>MGSSHHHHHHSSGLVPRGSHMPSYTVTVATGSQEHAGTDDYIYLSLVGSAGCSEKHLLDKGSFERGAVDSYDVTVDEELGEIQLVRIEKRKYGSNDDWYLKYITLKTPHGDYIEFPCYRWITGDVEVVLRDGRAKLARDDQIHILKQHRRKELETRQKQYRWMEWNPGFPLSIDAKCHKDLPRDIQFDSEKGVDFVLNYSKAMENLFINRFMHMFQSSWNDFADFEKIFVKISNTISERVMNHWQEDLMFGYQFLNGANPVLIRRCTELPEKLPVTTEMVECSLERQLSLEQEVQQGNIFIVDFELLDGIDANKTDPCTLQFLAAPICLLYKNLANKIVPIAIQLNQIPGDENPIFLPSDAKYDWLLAKIWVRSSDFHVHQTITHLLRTHLVSEVFGIAMYRQLPAVHPIFKLLVAHVRFTIAINTKAREQLICECGLFDKANATGGGGHVQMVQRAMKDLTYASLCFPEAIKARGMESKEDIPYYFYRDDGLLVWEAIRTFTAEVVDIYYEGDQVVEEDPELQDFVNDVYVYGMRGRKSSGFPKSVKSREQL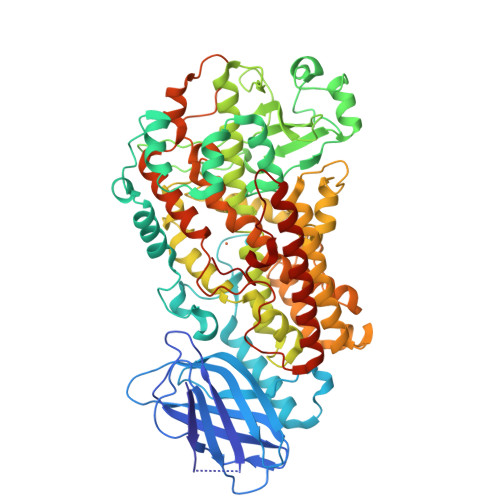SEYLTVVIFTASAQHAAVNFGQYDWASWIPNAPPTMRAPPPTAKGVVTIEQIVDTLPDRGRSCWHLGAVWALSQFQENELFLGMYPEEHFIEKPVKEAMARFRKNLEAIVSVIAERNENLQLPYYYLSPDRIPNSVAI[2x]3-(3-methyl-1H-pyrazol-5-yl)pyridine 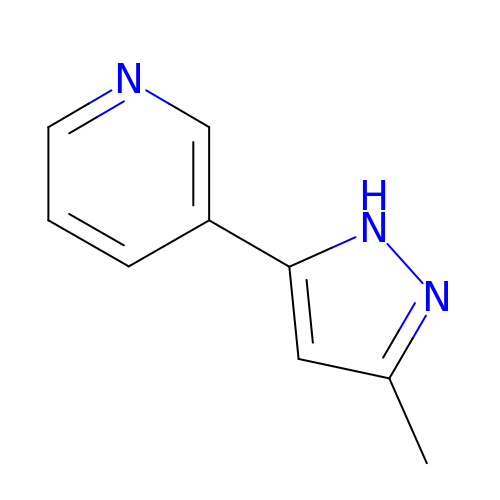| C9 H9 N3 | CGQOLRWLPQPKLV-UHFFFAOYSA-N>MANNSFITLNPSLPNSENSVIEAFSYKCIHCYNHHKFGTLEKLREAFPNLHFKLYPVSLMNGEFSKEMNELFAFAQYKDEQNGKDASYSDSLSHKLADVYFVSYFLNKQRNFSNLDEFYDIGLKAMNVNKNEVLNFLNTPKAKEILSEFQRANDI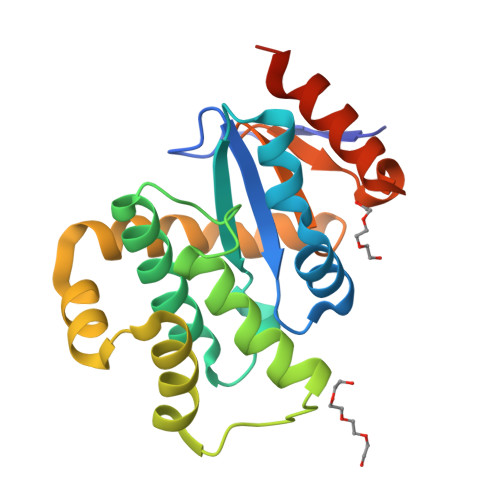AKTYGTPAFVVNGKYQINPSAINSMQDLEDLVKKLSNMKLEHHHHHH[2x]>GSGSKVLPKPLNAPNVIDTGHNFAVINISSEPYFGDGPIKSKKLLYKPVNHYEAWQHIQVTNEIVTLNYLEPRTEYELCVQLVRRGEGGEGHPGPVRRFTTASIGLPPPRGLNLLPKSQTTLNLTWQPIFPSSEDDF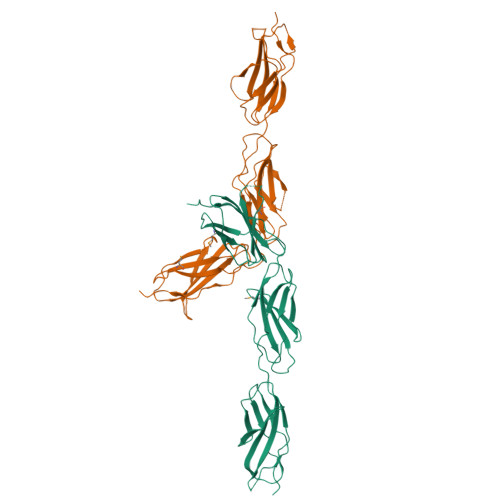YVEVERRSVQKSDQQNIKVPGNLTSVLLNNLHPREQYMVRARVNTKAQGEWSEDLTAWTLSDILPPQPENIKISNITHSSAMISWTILDGYSISSITIRYKVQGKNEDQHVDVKIKNATITQYQLKGLEPETAYQVDIFAENNIGSSNPAFSHELVTLPESQAPADL[2x]> MDPIINGNSANVYLTDSYLKGVISFSECNALGSYIFNGPYLKNDYTNLISRQNPLIEHMNLKKLNITQSLISKYHKGEIKLEEPTYFQSLLMTYKSMTSSEQIATTNLLKKIIRRAIEISDVKVYAILNKLGLKEKDKIKSNNGQDEDNSVITTIIKDDILSAVKDNQSHLKADKNHSTKQKDTIKTTLLKKLMCSMQHPPSWLIHWFNLYTKLNNILTQYRSNEVKNHGFTLIDNQTLSGFQFILNQYGCIVYHKELKRITVTTYNQFLTWKDISLSRLNVCLITWISNCLNTLNKSLGLRCGFNNVILTQLFLYGDCILKLFHNEGFYIIKEVEGFIMSLILNITEEDQFRKRFYNSMLNNITDAANKAQKNLLSRVCHTLLDKTVSDNIINGRWIILLSKFLKLIKLAGDNNLNNLSELYFLFRIFGHPMVDERQAMDAVKINCNETKFYLLSSLSMLRGAFIYRIIKGFVNNYNRWPTLRNAIVLPLRWLTYYKLNTYPSLLELTERDLIVLSGLRFYREFRLPKKVDLEMIINDKAISPPKNLIWTSFPRNYMPSHIQNYIEHEKLKFSESDKSRRVLEYYLRDNKFNECDLYNCVVNQSYLNNPNHVVSLTGKERELSVGRMFAMQPGMFRQVQILAEKMIAENILQFFPESLTRYGDLELQKILELKAGISNKSNRYNDNYNNYISKCSIITDLSKFNQAFRYETSCICSDVLDELHGVQSLFSWLHLTIPHVTIICTYRHAPPYIGDHIVDLNNVDEQSGLYRYHMGGIEGWCQKLWTIEAISLLDLISLKGKFSITALINGDNQSIDISKPIRLMEGQTHAQADYLLALNSLKLLYKEYAGIGHKLKGTETYISRDMQFMSKTIQHNGVYYPASIKKVLRVGPWINTILDDFKVSLESIGSLTQELEYRGESLLCSLIFRNVWLYNQIALQLKNHALCNNKLYLDILKVLKHLKTFFNLDNIDTALTLYMNLPMLFGGGDPNLLYRSFYRRTPDFLTEAIVHSVFILSYYTNHDLKDKLQDLSDDRLNKFLTCIITFDKNPNAEFVTLMRDPQALGSERQAKITSEINRLAVTEVLSTAPNKIFSKSAQHYTTTEIDLNDIMQNIEPTYPHGLRVVYESLPFYKAEKIVNLISGTKSITNILEKTSAIDLTDIDRATEMMRKNITLLIRILPLDCNRDKREILSMENLSITELSKYVRERSWSLSNIVGVTSPSIMYTMDIKYTTSTISSGIIIEKYNVNSLTRGERGPTKPWVGSSTQEKKTMPVYNRQVLTKKQRDQIDLLAKLDWVYASIDNKDEFMEELSIGTLGLTYEKAKKLFPQYLSVNYLHRLTVSSRPCEFPASIPAYRTTNYHFDTSPINRILTEKYGDEDIDIVFQNCISFGLSLMSVVEQFTNVCPNRIILIPKLNEIHLMKPPIFTGDVDIHKLKQVIQKQHMFLPDKISLTQYVELFLSNKTLKSGSHVNSNLILAHKISDYFHNTYILSTNLAGHWILIIQLMKDSKGIFEKDWGEGYITDHMFINLKVFFNAYKTYLLCFHKGYGKAKLECDMNTSDLLCVLELIDSSYWKSMSKVFLEQKVIKYILSQDASLHRVKGCHSFKLWFLKRLNVAEFTVCPWVVNIDYHPTHMKAILTYIDLVRMGLINIDRIHIKNKHKFNDEFYTSNLFYINYNFSDNTHLLTKHIRIANSELENNYNKLYHPTPETLENILANPIKSNDKKTLNDYCIGKNVDSIMLPLLSNKKLIKSSAMIRTNYSKQDLYNLFPMVVIDRIIDHSGNTAKSNQLYTTTSHQISLVHNSTSLYCMLPWHHINRFNFVFSSTGCKISIEYILKDLKIKDPNCIAFIGEGAGNLLLRTVVELHPDIRYIYRSLKDCNDHSLPIEFLRLYNGHINIDYGENLTIPATDATNNIHWSYLHIKFAEPISLFVCDAELSVTVNWSKIIIEWSKHVRKCKYCSSVNKCMLIVKYHAQDDIDFKLDNITILKTYVCLGSKLKGSEVYLVLTIGPANIFPVFNVVQNAKLILSRTKNFIMPKKADKESIDANIKSLIPFLCYPITKKGINTALSKLKSVVSGDILSYSIAGRNEVFSNKLINHKHMNILKWFNHVLNFRSTELNYNHLYMVESTYPYLSELLNSLTTNELKKLIKITGSLLYNFHNE;>MEKFAPEFHGEDANNRATKFLESIKGKFTSPKDPKKKDSIISVNSIDIEVTKESPITSNSTIINPTNETDDTAGNKPNYQRKPLVSFKEDPTPSDNPFSKLYKETIETFDNNEEESSYSYEEINDQTNDNITARLDRIDEKLSEILGMLHTLVVASAGPTSARDGIRDAMVGLREEMIEKIRTEALMTNDRLEAMARLRNEESEKMAKDTSDEVSLNPTSEKLNNLLEGNDSDNDLSLEDF[4x]

The respiratory syncytial virus (RSV) polymerase is a multifunctional RNA-dependent RNA polymerase composed of the large (L) protein and the phosphoprotein (P). It transcribes the RNA genome into ten viral mRNAs and replicates full-length viral genomic and antigenomic RNAs1. The RSV polymerase initiates RNA synthesis by binding to the conserved 3′-terminal RNA promoters of the genome or antigenome. The RSV L protein consists of five domains: the RdRp domain, the capping domain (Cap), the connector domain (CD), the methyltransferase domain (MT) and the carboxy-terminal domain (CTD).

The sequence of TrC10 is similar to that of Le10, except for the base composition at position 4: Le10 has a purine base G, whereas TrC10 has a pyrimidine base U. As a result, in the TrC10-bound RSV polymerase complex, we modelled the first 8 nt from the 3′ end of TrC10 RNA with the first 2 nt (T1U and T2G) in the catalytic pocket and the other 6 nt (T3C to T8U) in the template entrance channel. The T1U backbone of TrC10 interacts with residues R637, Q640 and G779 from the fingers region. T2G of TrC10 interacts with residues A541, K619, F629, A630 and E778. Among them, the T2G base of TrC10 has π–π interactions with F629. The polar oxygen and nitrogen atoms of the T2G base interact with residues K619 and E778. The remaining 6 nt of TrC10 are in the template entrance channel and interact with more than a dozen residues, including residues E620, R580, Y13, Y249, R747, S1155, E584, T551, R555, K570, E57, H229 and Y249. Comparing the TrC10- and Le10-bound RSV polymerase complexes, the visible 8 nt of TrC10 RNA correspond to positions 3–10 of the Le10 RNA. The twists occur at positions 3 and 6 in the TrC10-bound polymerase structure. We reveal that the polymerase prefers to initiate RNA synthesis at positions 3 of the Le10 promoter and 1 of the TrC10 promoter.> GGUCAAGAUAGUAAGGGUCCACGGUGGAUGCCCUGGCGCUGGAGCCGAUGAAGGACGCGAUUACCUGCGAAAAGCCCCGACGAGCUGGAGAUACGCUUUGACUCGGGGAUGUCCGAAUGGGGAAACCCACCUCGUAAGAGGUAUCCGCAAGGAUGGGAACUCAGGGAACUGAAACAUCUCAGUACCUGAAGGAGAAGAAAGAGAAUUCGAUUCCGUUAGUAGCGGCGAGCGAACCCGGAUCAGCCCAAACCGAAACGCUUGCGUUUCGGGGUUGUAGGACCAGUUUUUAAGAUUCAACCCCUCAAGCCGAAGUGGCUGGAAAGCUACACCUCAGAAGGUGAGAGUCCUGUAGGCGAACGAGCGGUUGACUGUACUGGCACCUGAGUAGGUCGUUGUUCGUGAAACGAUGACUGAAUCCGCGCGGACCACCGCGCAAGGCUAAAUACUCCCAGUGACCGAUAGCGCAUAGUACCGUGAGGGAAAGGUGAAAAGAACCCCGGGAGGGGAGUGAAAGAGAACCUGAAACCGUGGACUUACAAGCAGUCAUGGCACCUUAUGCGUGUUAUGGCGUGCCUAUUGAAGCAUGAGCCGGCGACUUAGACCUGACGUGCGAGCUUAAGUUGAAAAACGGAGGCGGAGCGAAAGCGAGUCCGAAUAGGGCGGCAUUAGUACGUCGGGCUAGACUCGAAACCAGGUGAGCUAAGCAUGACCAGGUUGAAACCCCCGUGACAGGGGGCGGAGGACCGAACCGGUGCCUGCUGAAACAGUCUCGGAUGAGUUGUGUUUAGGAGUGAAAAGCUAACCGAACCUGGAGAUAGCUAGUUCUCCCCGAAAUGUAUUGAGGUACAGCCUCGGAUGUUGACCAUGUCCUGUAGAGCACUCACAAGGCUAGGGGGCCUACCAGCUUACCAAACCUUAUGAAACUCCGAAGGGGCACGCGUUUAGUCCGGGAGUGAGGCUGCGAGAGCUAACUUCCGUAGCCGAGAGGGAAACAACCCAGACCAUCAGCUAAGGUCCCUAAAUGAUCGCUCAGUGGUUAAGGAUGUGUCGUCGCAUAGACAGCCAGGAGGUUGGCUUAGAAGCAGCCACCCUUCAAAGAGUGCGUAAUAGCUCACUGGUCGAGUGACGAUGCGCCGAAAAUGAUCGGGGCUCAAGUGAUCUACCGAAGCUAUGGAUUCAACUCGCGAAGCGAGUUGUCUGGUAGGGGAGCGUUCAGUCCGCGGAGAAGCCAUACCGGAAGGAGUGGUGGAGCCGACUGAAGUGCGGAUGCCGGCAUGAGUAACGAUAAAAGAAGUGAGAAUCUUCUUCGCCGUAAGGACAAGGGUUCCUGGGGAAGGGUCGUCCGCCCAGGGAAAGUCGGGACCUAAGGUGAGGCCGAACGGCGCAGCCGAUGGACAGCAGGUCAAGAUUCCUGCACCGAUCAUGUGGAGUGAUGGAGGGACGCAUUACGCUAUCCAAUGCCAAGCUAUGGCUAUGCUGGUUGGUACGCUCAAGGGCGAUCGGGUCAGAAAAUCUACCGGUCACAUGCCUCAGACGUAUCGGGAGCUUCCUCGGAAGCGAAGUUGGAAACGCGACGGUGCCAAGAAAAGCUUCUAAACGUUGAAACAUGAUUGCCCGUACCGCAAACCGACACAGGUGUCCGAGUGUCAAUGCACUAAGGCGCGCGAGAGAACCCUCGUUAAGGAACUUUGCAAUCUCACCCCGUAACUUCGGAAGAAGGGGUCCCCACGCUUCGCGUGGGGCGCAGUGAAUAGGCCCAGGCGACUGUUUACCAAAAUCACAGCACUCUGCCAACACGAACAGUGGACGUAUAGGGUGUGACGCCUGCCCGGUGCCGGAAGGUCAAGUGGAGCGGUGCAAGCUGCGAAAUGAAGCCCCGGUGAACGGCGGCCGUAACUAUAACGGUCCUAAGGUAGCGAAAUUCCUUGUCGGGUAAGUUCCGACCUGCACGAAAGGCGUAACGAUCUGGGCGCUGUCUCAACGAGGGACUCGGUGAAAUUGAAUUGGCUGUAAAGAUGCGGCCUACCCGUAGCAGGACGAAAAGACCCCGUGGAGCUUUACUAUAGUCUGGCAUUGGGAUUCGGGUUUCUCUGCGUAGGAUAGGUGGGAGCCUGCGAAACUGGCCUUUUGGGGUCGGUGGAGGCAACGGUGAAAUACCACCCUGAGAAACUUGGAUUUCUAACCUGAAAAAUCACUUUCGGGGACCGUGCUUGGCGGGUAGUUUGACUGGGGCGGUCGCCUCCCAAAAUGUAACGGAGGCGCCCAAAGGUCACCUCAAGACGGUUGGAAAUCGUCUGUAGAGCGCAAAGGUAGAAGGUGGCUUGACUGCGAGACUGACACGUCGAGCAGGGAGGAAACUCGGGCUUAGUGAACC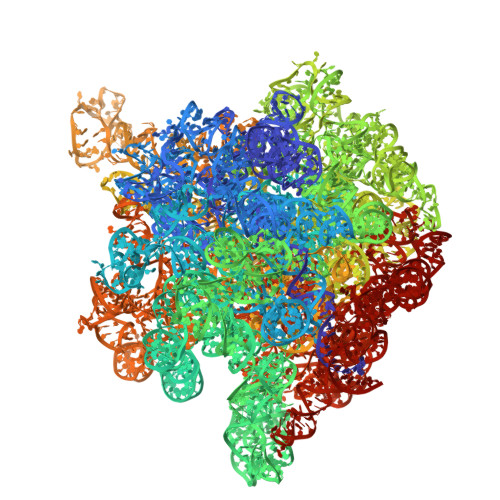GGUGGUACCGUGUGGAAGGGCCAUCGAUCAACGGAUAAAAGUUACCCCGGGGAUAACAGGCUGAUCUCCCCCGAGAGUCCAUAUCGGCGGGGAGGUUUGGCACCUCGAUGUCGGCUCGUCGCAUCCUGGGGCUGAAGAAGGUCCCAAGGGUUGGGCUGUUCGCCCAUUAAAGCGGCACGCGAGCUGGGUUCAGAACGUCGUGAGACAGUUCGGUCUCUAUCCGCUACGGGCGCAGGAGAAUUGAGGGGAGUUGCUCCUAGUACGAGAGGACCGGAGUGAACGGACCGCUGGUCUCCCUGCUGUCGUACCAACGGCACAUGCAGGGUAGCUAUGUCCGGAACGGAUAACCGCUGAAAGCAUCUAAGCGGGAAGCCAGCCCCAAGAUGAGUUCUCCCACUGUUUAUCAGGUAAGACUCCCGGAAGACCACCGGGUUAAGAGGCCAGGCGUGCACGCAUAGCAAUGUGUUCAGCGGACUGGUGCUCAUCAGUCGAGGUCUUGACCACUC> PVSEKQLAEVVA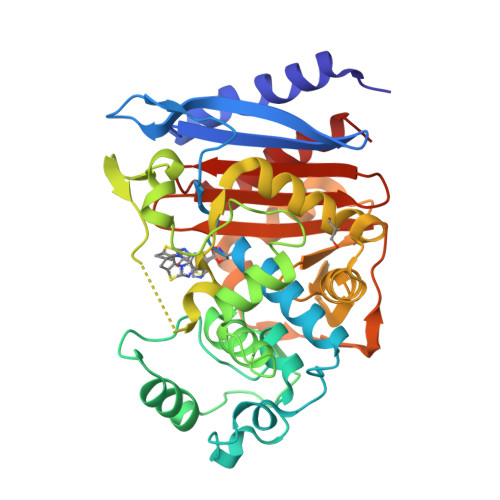NTVTPLMKAQSVPGMAVAVIYQGKPHYYTFGKADIAANKPVTPQTLFELGSISKTFTGVLGGDAIARGEISLDDPVTRYWPQLTGKQWQGIRMLDLATYTAGGLPLQVPDEVTDNASLLRFYQNWQPQWKPGTTRLYANASIGLFGALAVKPSGMPYEQAMTTRVLKPLKLDHTWINVPKAEEAHYAWGYRDGKAVRAVRVSPGMLDAQAYGVKTNVQDMANWVMANMAPENVADASLKQGIALAQSRYWRIGSMYQGLGWEMLNWPVEANTVVEGSDSKVALAPLPVAEVNPPAPPVKASWVHKTGSTGGFGSYVAFIPEKQIGIVMLANTSYPNPARVEAAYHILEALQ> MFKDGSLIPYLTAGDPDKQSTLNFLLALDEYAGAIELGIPFSDPIADGKTIQESHYRALKNGFKLREAFWIVKEFRRHSSTPIVLMTYYNPIYRAGVRNFLAEAKASGVDGILVVDLPVFHAKEFTEIAREEGIKTVFLAAPNTPDERLKVIDDMTTGFVYLVSLYGTTGAREEIPKTAYDLLRRAKRICRNKVAVGFGVSKREHVVSL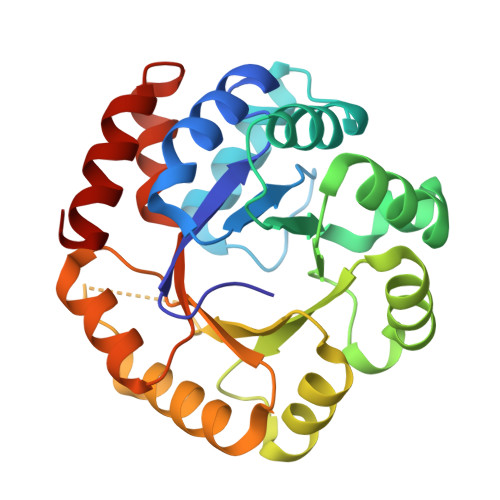LKEGANGVVVGSALVKIIGEKGREATEFLKKKVEELLGI>[2x]MKTIGLVISTLNNPFFVTLKNGAEEKAKELGYKIIVEDSQNDSSKELSNVEDLIQQKVDVLLINPVDSDAVVTAIKEANSKNIPVITIDRSANGGDVVCHIASDNVKGGEMAAEFIAKALKGKGNVVELEGIPGASAARDRGKGFDEAIAKYPDIKIVAKQAADFDRSKGLSVMENILQAQPKIDAVFAQNDEMALGAIKAIEAANRQGIIVVGFDGTEDALKAIKEGKMAATIAQQPALMGSLGVEMADKYLKGEKIPNFIPAELKLITKENVQGSHHHHHH

The ribose-binding proteins are members of the periplasmic binding protein (PBP) superfamily whose members play roles in prokaryotic ABC transport, chemotaxis, and intercellular communication systems. The PBP fold consists of two domains each of which adopts a three-layered α/β/α sandwich motif. The two domains are linked by two or three β-strands that form a flexible hinge which permits the domains of the protein to bend towards each other in response to ligand binding at the interface between the two domains. Here we report the high-resolution X-ray crystallographic structure of a ribose binding protein (tteRBP) from the hyperthermophilic bacterium T. tengcongensis (optimal growth temp ~80°C).

The tteRBP crystal structure was solved to 1.9 Å resolution by molecular replacement using the ribose-bound form of ecRBP as the search model. The asymmetric unit contains 346 water molecules and two tteRBP molecules (residues 40–313) in essentially identical conformations (0.12 Å RMSD of backbone atoms) complexed with ribose. The tteRBP structure adopts the overall fold and topology that is characteristic of periplasmic ribose-binding proteins. The apparent thermal transition midpoint (appTm) of 102°C in the absence of GdCl was determined by linear extrapolation of a series of melting point determinations carried out at different GdCl concentrations. tteRBP is therefore significantly more stable than the mesophilic ecRBP (appTmvalue is 56°C). The appTm value of the ribose complex in the absence of GdCl is 114°C; the appTm value for ecRBP under equivalent conditions is 72°C. Analysis of main-chain and side-chain geometry of the aligned structures indicates there are few differences in the main-chain geometries of ecRBP and tteRBP (0.4 Å RMSD of 235/271 Cα positions and 0.65 Å RMSD of 270/271 Cα positions and distance between aligned Cα positions range from 0.03–3.1 Å over 270 Cα positions). The loops and turns in the binding pocket retain near-identical conformations. Polar amino acids, non-polar amino acids, waters, and the hydrogen-bonding interactions are identical in both tteRBP and ecRBP sugar-binding pockets. A bias is observed for a gain of polar and charged amino acids on the surface of tteRBP (net of twelve charged and three polar substitutions), while the opposite is observed for the tteRBP core, where there is a bias for the loss of polar amino acids (seven net substitutions). The comparative analysis presented here shows that the substitutions responsible for conferring thermal stability on tteRBP are encoded in side-chain identity and location (core, boundary or surface) which serves to alter surface polarity/charge, removal of unsatisfied core hydrogen bonds and increase in core/boundary side-chain hydrophobicity.>[2x]MVRV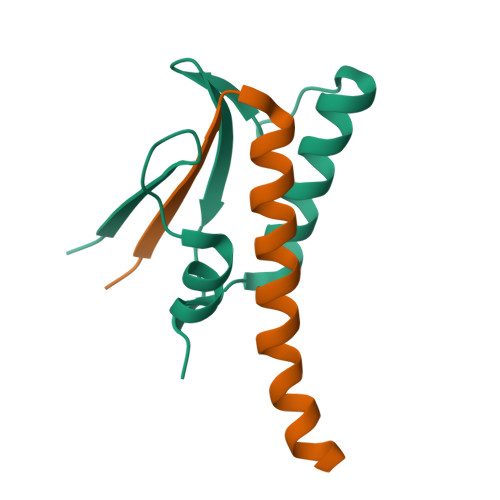TSAKEESIDVDSSSYISAENLAKKYVFNPKEVSEAYNAIVALQNDGIESDLVQLVNGKYQVIFYPEGKRLETKS;>MADIIADADSPAKITIKANKLKDLKDYVDDLKTYNNTYSNVVLEHHHHHH[2x]>DEEASGAETTSGIPDLDSLPPTYSAMCPFGCHCHLRVVQCSDLGLKAVPKEISPDTTLLDLQNNDISELRKDDFKGLQHLYALVLVNNKISKIHEKAFSPLRKLQKLYISKNHLVEIPPNLPSSLVELRIHDNRIRKVPKGVFSGLRNMNCIEMGGNPLENSGFEPGAFDGLKLNYLRISEAKLTGIPKDLPETLNELHLDHNKIQAIELEDLLRYSKLYRLGLGHNQIRMIENGSLSFLPTLRELHLDNNKLSRVPAGLPDLKLLQVVYLHTNNITKVGVNDFCPVGFGVKRAYYNGISLFNNPVPYWEVQPATFRC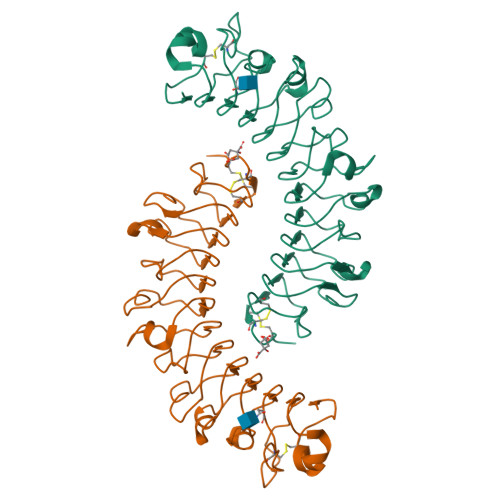VTDRLAIQFGNYKK[6x]>MDYKDDDDKAAHRPVEWVQAVVSRFDEQLPIKTGQQNTHTKVSTEHNKECLINISKYKFSLVISGLTTILKNVNNMRIFGEAAEKNLYLSQLIILDTLEKCLAGQPKDTMRLDETMLVKQLLPEICHFLHTCREGNQHAAELRNSASGVLFSLSCNNFNAVFSRISTRLQELTVCSEDNVDVHDIELLQYINVDCAKLKRLLKETAFKFKALKKVAQLAVINSLEKAFWNWVENYPDEFTKLYQIPQTDMAECAEKLFDLVDGFAESTKRKAAVWPLQIILLILCPEIIQDISKDVVDENNMNKKLFLDSLRKALAGHGGSRQLTESAAIACVKLCKASTYINWEDNSVIFLLVQSMVVDLKNLLFNPSKPFSRGSQPADVDLMIDCLVSCFRISPHNNQHFKICLAQNSPSTFHYVLVNSLHRIITNSALDWWPKIDAVYCHSVELRNMFGETLHKAVQGCGAHPAIRMAPSLTFKEKVTSLKFKEKPTDLETRSYKYLLLSMVKLIHADPKLLLCNPRKQGPETQGSTAELITGLVQLVPQSHMPEIAQEAMEALLVLHQLDSIDLWNPDAPVETFWEISSQMLFYICKKLTSHQMLSSTEILKWLREILICRNKFLLKNKQADRSSCHFLLFYGVGCDIPSSGNTSQMSMDHEELLRTPGASLRKGKGNSSMDSAAGCSGTPPICRQAQTKLEVALYMFLWNPDTEAVLVAMSCFRHLCEEADIRCGVDEVSVHNLLPNYNTFMEFASVSNMMSTGRAALQKRVMALLRRIEHPTAGNTEAWEDTHAKWEQATKLILNYPKAKMEDGQAAESLHKTIVKRRMSHVSGGGSIDLSDTDSLQEWINMTGFLCALGGVCLQQRSNSGLATYSPPMGPVSERKGSMISVMSSEGNADTPVSKFMDRLLSLMVCNHEKVGLQIRTNVKDLVGLELSPALYPMLFNKLKNTISKFFDSQGQVLLTDTNTQFVEQTIAIMKNLLDNHTEGSSEHLGQASIETMMLNLVRYVRVLGNMVHAIQIKTKLCQLVEVMMARRDDLSFCQEMKFRNKMVEYLTDWVMGTSNQAADDDVKCLTRDLDQASMEAVVSLLAGLPLQPEEGDGVELMEAKSQLFLKYFTLFMNLLNDCSEVEDESAQTGGRKRGMSRRLASLRHCTVLAMSNLLNANVDSGLMHSIGLGYHKDLQTRATFMEVLTKILQQGTEFDTLAETVLADRFERLVELVTMMGDQGELPIAMALANVVPCSQWDELARVLVTLFDSRHLLYQLLWNMFSKEVELADSMQTLFRGNSLASKIMTFCFKVYGATYLQKLLDPLLRIVITSSDWQHVSFEVDPTRLEPSESLEENQRNLLQMTEKFFHAIISSSSEFPPQLRSVCHCLYQVVSQRFPQNSIGAVGSAMFLRFINPAIVSPYEAGILDKKPPPRIERGLKLMSKILQSIANHVLFTKEEHMRPFNDFVKSNFDAARRFFLDIASDCPTSDAVNHSLSFISDGNVLALHRLLWNNQEKIGQYLSSNRDHKAVGRRPFDKMATLLAYLGPPEHKPVADTHWSSLNLTSSKFEEFMTRHQVHEKEEFKALKTLSIFYQAGTSKAGNPIFYYV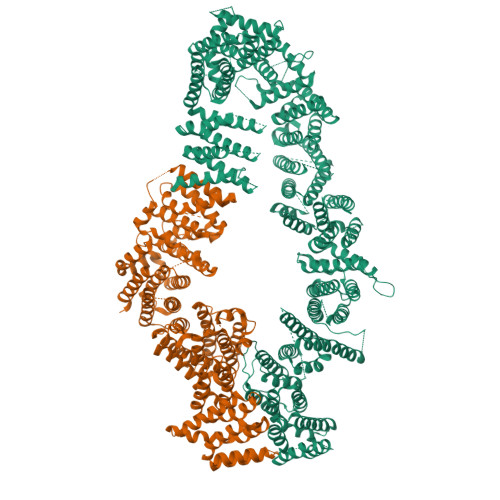ARRFKTGQINGDLLIYHVLLTLKPYYAKPYEIVVDLTHTGPSNRFKTDFLSKWFVVFPGFAYDNVSAVYIYNCNSWVREYTKYHERLLTGLKGSKRLVFIDCPGKLAEHIEHEQQKLPAATLALEEDLKVFHNALKLAHKDTKVSIKVGSTAVQVTSAERTKVLGQSVFLNDIYYASEIEEICLVDENQFTLTIANQGTPLTFMHQECEAIVQSIIHIRTRWELSQPDSIPQHTKIRPKDVPGTLLNIALLNLGSSDPSLRSAAYNLLCALTCTFNLKIEGQLLETSGLCIPANNTLFIVSISKTLAANEPHLTLEFLEECISGFSKSSIELKHLCLEYMTPWLSNLVRFCKHNDDAKRQRVTAILDKLITMTINEKQMYPSIQAKIWGSLGQITDLLDVVLDSFIKTSATGGLGSIKAEVMADTAVALASGNVKLVSSKVIGRMCKIIDKTCLSPTPTLEQHLMWDDIAILARYMLMLSFNNSLDVAAHLPYLFHVVTFLVATGPLSLRASTHGLVINIIHSLCTCSQLHFSEETKQVLRLSLTEFSLPKFYLLFGISKVKSAAVIAFRSSYRDRSFSPGSYERETFALTSLETVTEALLEIMEACMRDIPTCKWLDQWTELAQRFAFQYNPSLQPRALVVFGCISKRVSHGQIKQIIRILSKALESCLKGPDTYNSQVLIEATVIALTKLQPLLNKDSPLHKALFWVAVAVLQLDEVNLYSAGTALLEQNLHTLDSLRIFNDKSPEEVFMAIRNPLEWHCKQMDHFVGLNFNSNFNFALVGHLLKGYRHPSPAIVARTVRILHTLLTLVNKHRNCDKFEVNTQSVAYLAALLTVSEEVRSRCSLKHRKSLLLTDISMENVPMDTYPIHHGDPSYRTLKETQPWSSPKGSEGYLAATYPTVGQTSPRARKSMSLDMGQPSQANTKKLLGTRKSFDHLISDTKAPKRQEMESGITTPPKMRRVAETDYEMETQRISSSQQHPHLRKVSVSESNVLLDEEVLTDPKIQALLLTVLATLVKYTTDEFDQRILYEYLAEASVVFPKVFPVVHNLLDSKINTLLSLCQDPNLLNPIHGIVQSVVYHEESPPQYQTSYLQSFGFNGLWRFAGPFSKQTQIPDYAELIVKFLDALIDTYLPGIDEETSEESLLTPTSPYPPALQSQLSITANLNLSNSMTSLATSQHSPGIDKENVELSPTTGHCNSGRTRHGSASQVQKQRSAGSFKRNSIKKIV[2x]> AEAGITGTWYAQLGDTFIVTAGADGALTGTYEAAVGDDDGDDDGDDDGAESRYVLTGRYDSAPATDGSGTALGWTVAWKNNYRNAHSATTWSGQYVGGAEARINTQWLLTSGTTEANAWKSTLVGHDTF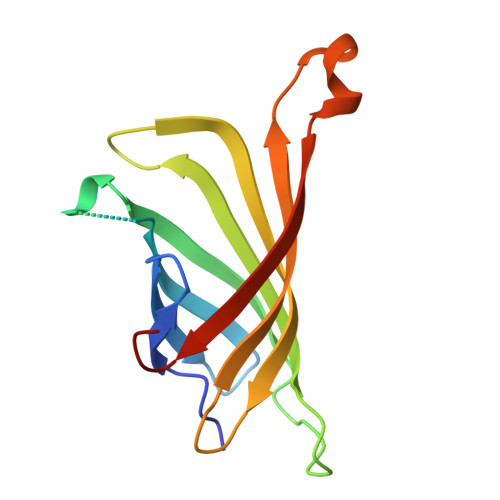TKVKPSAAS>TQPALLRLSDHLLANYKKGVRPVRDWRKPTTVSIDVIMYAILNVDEKNQVLTTYIWYRQYWTDEFLQWTPEDFDNVTKLSIPTDSIWVPDILINEFVDVGKSPNIPYVYVHHRGEVQNYKPLQLVTACSLDIYNFPFDVQNCSLTFTSWLHTIQDINITLWRSPEEVRSDKSIFINQGEWELLEVFPQFKEFSIDISNSYAEMKFYVIIRRRPLFYAVSLLLPSIFLMVVDIVGFCLPPDSGERVSFKITLLLGYSVFLIIVSDTLPATAIGTPLIGVYFVVCMALLVISL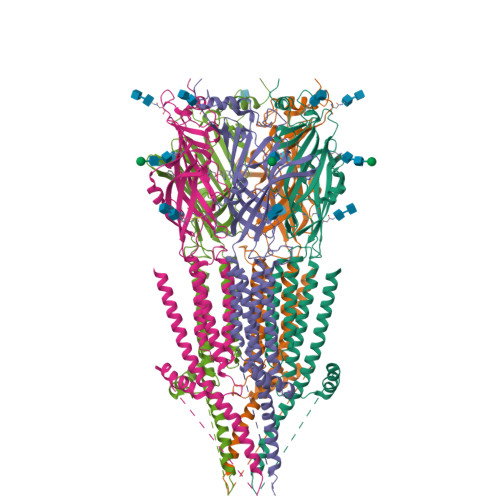AETIFIVRLVHKQDLQRPVPDWLRHLVLDRIAWILCLGEQPMAHRPPATFQANKTDDCSGSDLLPAMGNHCSHVGGPQDLEKTPRGRGSPLPPPREASLAVRGLLQELSSIRHFLEKRDEMREVARDWLRVGYVLDRLLFRIYLLAVLAYSITLVTLWSI[5x]>DHYNCVSSGGQCLYSACPIFTKIQGTCYRGKAKCCK[2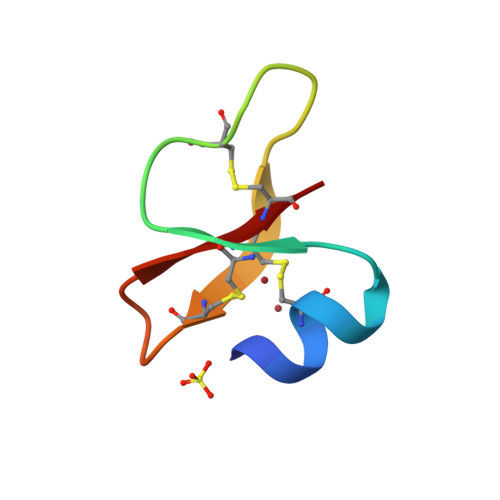x]>MLHILCQGTPFEIGYEHGSAAKAVIARSIDFAVDLIRGKTKKTDEELKQVLSQLGRVIEERWPKYYEEIRGIAKGAERDVSEIVMLNTRTEFAYGLKAARDGATTAYCQLPNGALQGQNWDFFSATKENLIRLTIRQAGLPTIKFITEAGIIGKVGFNSAGVAVNYNALHLQGLRPTGVPSHIALRIALESTSPSQAYDRIVEQGGMAASAFIMVGNGHEAFGLEFSPTSIRKQVLDANGRMVHTNHCLLQHGKNEKELDPLPDSWNRHQRMEFLLDGFDGTKQAFAQLWADEDNYPFSICRAYEEGKSR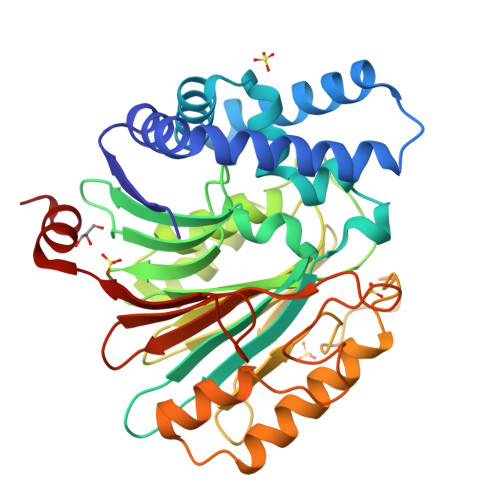GATLFNIIYDHARREATVRLGRPTNPDEMFVMRFDEEDERSALNARL[4x]N~2~-(morpholin-4-ylcarbonyl)-N-[(3S)-1-phenyl-5-(phenylsulfonyl)pentan-3-yl]-L-leucinamide | C28 H39 N3 O5 S | 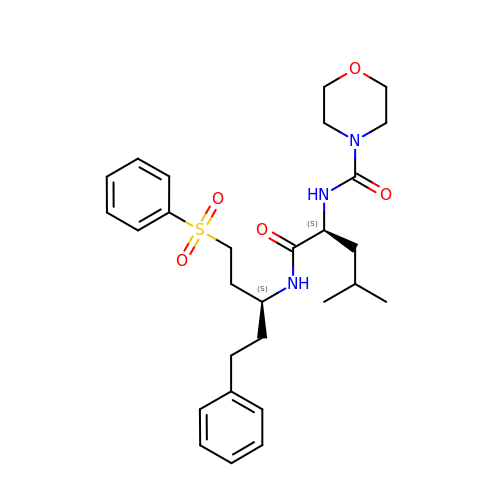IHIAYQGDASIWGA-AHWVRZQESA-N Here we identify and characterise a sub-family of multi-centre photoreceptors, termed photocobilins, that use B12 and biliverdin (BV) to sense light across the visible spectrum. We have identified and characterised two types of photocobilins, one from Saccharothrix syringae (SasPcob) that represents a standalone photocobilin photoreceptor and a more complex protein that consists of a photocobilin diguanylate cyclase (DGC) fusion from Acidimicrobiaceae bacterium (AbDPcob) that is representative of a photocobilin domain fused to an enzyme domain. Crystal structures reveal close juxtaposition of the B12 and BV chromophores, an arrangement that facilitates optical coupling. Light-triggered conversion of the B12 affects quaternary structure, in turn leading to light-activation of associated enzyme domains.

In order to investigate the effects of illumination on the photocobilins, we determined the light-exposed SasPcob crystal structure. Similar to CarH, the SasPcob light state corresponds to a monomeric species, with the B12-binding domain dimer interface disrupted by the light-triggered release of the adenosine group (Fig. 7 and Supplementary Figs. 10−21). However, the SasPcob light state structure lacks the drastic large-scale domain repositioning that accompanies formation of a bis-His ligated cobalamin in CarH. Instead, more modest changes occur at the adenosine binding pocket in SasPcob culminating with the formation of a water/hydroxide ligated Co(III)balamin. While the majority of the Rossmann and globin binding domains are relatively unperturbed, the N-terminal four helix bundle adapts to the removal of the adenosine through changes in the position of the Glu71/His72 containing helix. The C-alpha displacement of ~2.4 Å at the Glu71/His72 region is such that, when superposed on the corresponding dark SasPcob dimer, it would lead to a severe clash at the dimer interface. Therefore, we postulate that rearrangement of the adenosine binding pocket in response to illumination occurs concomitantly with monomer formation.

> VDILAAGREELMAALAEGDEHAAVDLAMRLLDGGVPADVVLLELVADAQVEIGVLWQANRWSVAQEHAATAISERVIAAVGDRAAAAPTRGHVVVACLDGEWHALPARIVAEVLRGRGWRVTFLGASVPAAHLVPYLEEHGPDAVALSCTLPRGLPRADQVVAACRATGTPVLVGGLGFGPDGRWARVLGAGTWAPTARAAADLLDRPEWPRTALPAPPRPADPEYAALRARRAELVDAGLAALHEWFPPLRDYDARRLDATLDDLGDIVDHLAASVYVDDPELFGEFVTWTAEVLAARGVSPASVEVALEAIARVLDDHPRTRHHLDHGRRALAAHLEHH> AMHPRKDWYELTRATNWTPSYVTEEQLFPERMSGHMGIPLEKWESYDEPYKTSYPEYVSIQREKDAGAYSVKAALERAKIYENSDPGWISTLKSHYGAIAVLEYAAVTGEGRMARFSKAPGNRNMATFGMMDELRHGQLQLFFPHEYCKKDRQFDWAWRAYHSNEWAAIAAKHFFDDIITGRDAISVAIMLTFSFETGFTNMQFLGLAADAAEAGDYTFANLISSIQTDESRHAQQGGPALQLLIENGKREEAQKKVDMAIWRAWRLFAVLTGPVMDYYTPLEDRSQSFKEFMYEWIIGQFERSLIDLGLDKPWYWDLFLKDIDELHHSYHMGVWYWRTTAWWNPAAGVTPEERDWLEEKYPGWNKRWGRCWDVIT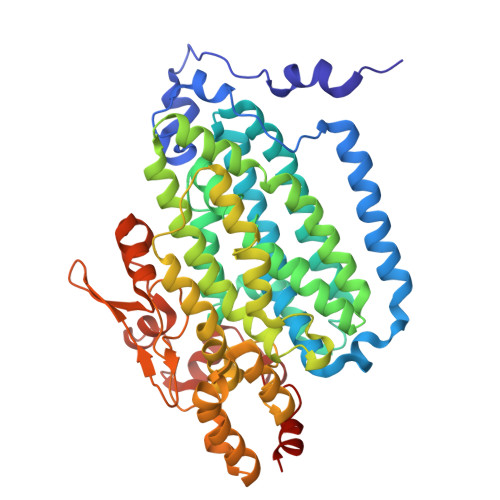ENVLNDRMDLVSPETLPSVCNMSQIPLVGVPGDDWNIEVFSLEHNGRLYHFGSEVDRWVFQQDPVQYQNHMNIVDRFLAGQIQPMTLEGALKYMGFQSIEEMGKDAHDFAWADKCK> TVKWIEAVALSDILEGDVLGVTVEGKELALYEVEGEIYATDNLCTHGSARMSDGYLEGREIECPLHQGRFDVCTGKA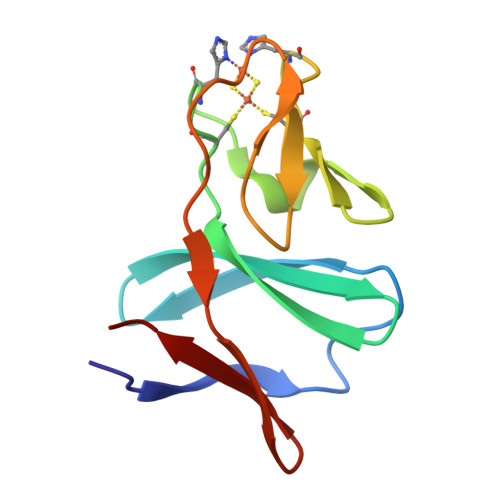LCAPVTQNIKTYPVKIENLRVMIDLS> MEEFQQIPDFYGCYLLQSISKRQSFYIGSTPNPVRRLRQHNGSLSRGGAYRTKRDGTRPWEMVAIVYGFPSRIAALQFQHAWQHGYQTRYIKSQDRVVKTRKGGRSIHHKLAMITSLLKNEYFRYMDLTLHFFNQKVEEIWKNDKFNVSQTQESIDNNYTVSLSQDALTEINNDTI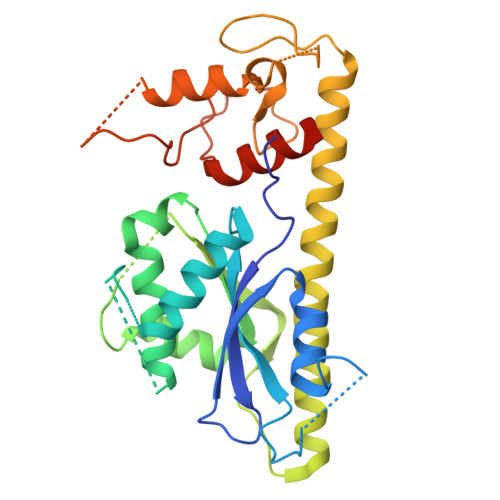DDIMDVNEKNMELVQNLYSTTLAEKTKTLLLYKEKIDTGINTCQFCNKIIKHNLSGNISENLFAFCRDTSCTFVSHLACAYRYFMSNTELPKEDTIIPQSPKCPKCYTLLKWCDVIYYSIKLNKDNTTADDKKKTI>[6x]MFSKFFIERPVFASVVAIIISLAGAIGLTNLPIEQYPSLTPPTVKVSATYTGADAQTIASTVASPIEDAINGADNMIYMDSTSSSSGTMSLTVYFDIGTDPDQATIDVNNRISAATAKMPDAVKKLGVTVRKTSSTTLAAISMYSSDGSMSAVDVYNYITLNVLDELKRVPGVGDANAIGNRNYSLRIWLKPDLLNKFGITATDVISAVNDQNAQYATGKIGEEPVTQKSPYVY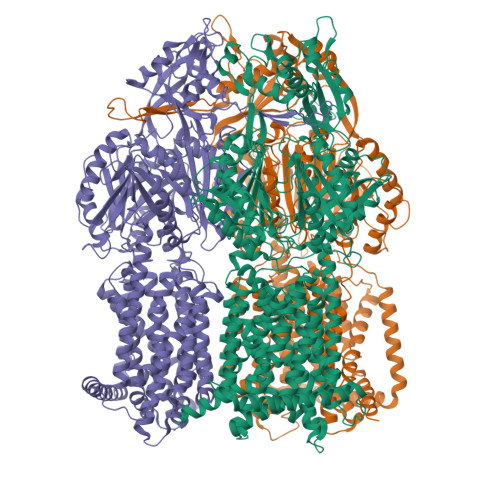SITMQGRLQNPSEFENIILRTNNDGSFLRLKDVADVEIGSQQYSSQGRLNGNDAVPIMINLQSGANALHTAELVQAKMQELSKNFPKGLTYKIPYDTTKFVIESIKEVVKTFVEALILVIIVMYMFLKNFRATLIPMIAVPVSLLGTFAGLYVLGFSINLLTLFALILAIGIVVDDAIIVVENIDRILHENEQISVKDAAIQAMQEVSSPVISIVLVLCAVFVPVSFISGFVGEIQRQFALTLAISVTISGFVALTLTPSLCALFLRRNEGEPFKFVKKFNDFFDWSTSVFSAGVAYILKRTIRFVLIFCIMLGAIFYLYKAVPNSLVPEEDQGLMISIINLPSASALHRTISEVDHISQEVLKTNGVKDAMAMIGFDLFTSSLKENAAAMFIGLQDWKDRNVSADQIIAELNKKFAFDRNASSVFIGLPPIPGLSITGGFEMYVQNKSGKSYDEIQKDVNKLVAAANQRKELSRVRTTLDTTFPQYKLIIDRDKLKHYNLNMQDVFNTMNATIGTYYVNDFSMLGKNFQVNIRAKGDFRNTQDALKNIFVRSNDGKMIPLDSFLTLQRSSGPDDVKRFNLFPAAQVQGQPAPGYTSGQAIEAIAQVAKETLGDDYSIAWSGSAYQEVSSKGTASYAFALGMIFVFLILAAQYERWLIPLAVVTAVPFAVFGSFLLVYLRGFSNDIYFQTGLLLLIGLSAKNAILIVEFAMEERFKKGKGVFEAAVAAAKLRFRPIIMTSLAFTFGVLPMIFATGAGSASRHSLGTGLIGGMIAASTLAIFFVPLFFYLLENFNEWLDKKR> MGAQVSTQKSGSHETGNVATGGSTINFTNINYYKDSYAASATRQDFTQDPKKFTQPVLDSIRELSAPLNSPSVEACGYSDRVAQLTVGNSSITTQEAANIVLAYGEWPEYCPDTDATAVDKPTRPDVSVNRFYTLDSKMWQENSTGWYWKFPDVLNKTGVFGQNAQFHYLYRSGFCLHVQCNASKFHQGALLVAVIPEFVIAGRGSNTKPNEAPHPGFTTTFPGTTGATFYDPYVLDSGVPLSQALIYPHQWINLRTNNCATVIV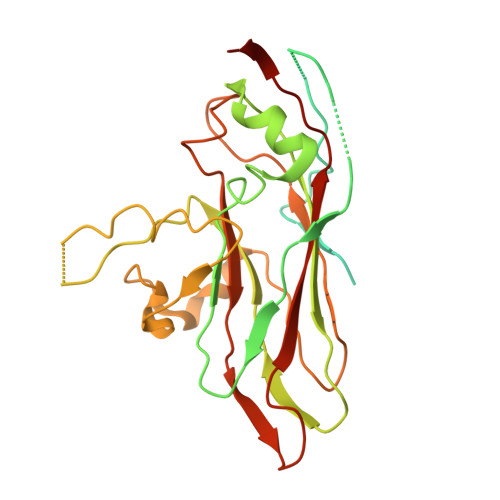PYINAVPFDSAINHSNFGLIVIPVSPLKYSSGATTAIPITITIAPLNSEFGGLRQAVSQ> MELGPAEPMVVVPVDVEKEDVRILKVCFYSNSFNPGKNFKLVKCTVQTEIREIITSILLSGRIGPNIRLAECYGLRLKHMKSDEIHWLHPQMTVGEVQDKYECLHVEAEWRYDLQIRYLPEDFMESLKEDRTTLLYFYQQLR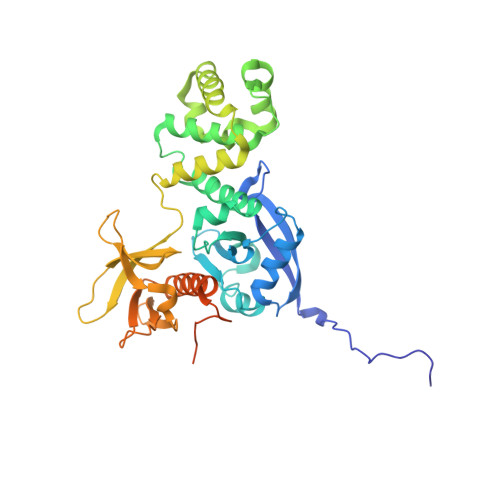NDYMQRYASKVSEGMALQLGCLELRRFFKDMPHNALDKKSNFELLEKEVGLDLFFPKQMQENLKPKQFRKMIQQTFQQYASLREEECVMKFFNTLAGFANIDQETYRCELIQGWNITVDLVIGPKGIRQLTSQDAKPTCLAEFKQIRSIRCLPLEEGQAVLQLGIEGAPQALSIKTSSLAEAENMADLIDGYCRLQGEHQGSLIIHPRKDGEKRNSLPQIPMLNLEARRSHLSESCSIESDIYAEIPDET>ELTPDQQTLLHFIMDSYNKQRMPQEITNKILKEEFSAEENFLILTEMATNHVQVLVEFTKKLPGFQTLDHEDQIALLKGSAVEAMFLRSAEIFNKKLPSGHSDLLEERIRNSGISDEYITPMFSFYKSIGELKMTQEEYALLTAIVILSPDRQYIKDREAVEKLQEPLLDVLQKLCKI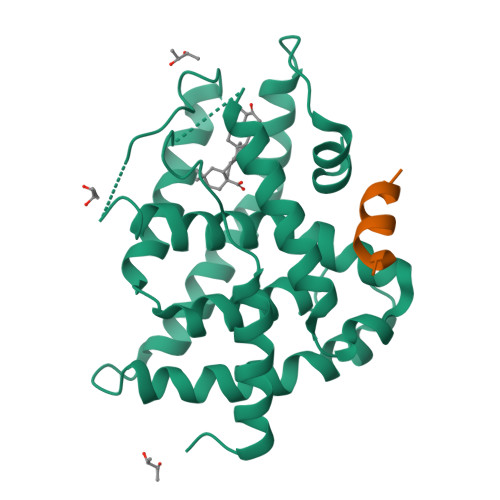HQPENPQHFACLLGRLTELRTFNHHHAEMLMSWRVNDHKFTPLLCEIWDV[2x];>ENALLRYLLDKD[2x]>[2x]MSALVLKPCAAVSIRGSSCRARQVAPRAPLAASTVRVALATLEAPARRLGNVACAAAAPAAEAPLSHVQQALAELAKPKDDPTRKHVCVQVAPAVRVAIAETLGLAPGATTPKQLAEGLRRLGFDEVFDTLFGADLTIMEEGSELLHRLTEHLEAHPHSDEPLPMFTSCCPGWIAMLEKSYPDLIPYVSSCKSPQMMLAAMVKSYLAEKKGIAPKDMVMVSIMPCTRKQSEADRDWFCVDADPTLRQLDHVITTVELGNIFKERGINLAELPEGEWDNPMGVGSGAGVLFGTTGGVMEAALRTAYELFTGTPLPRLSLSEVRGMDGIKETNITMVPAPGSKFEELLKH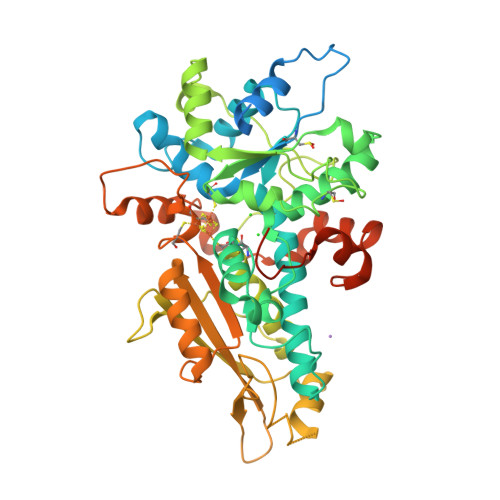RAAARAEAAAHGTPGPLAWDGGAGFTSEDGRGGITLRVAVANGLGNAKKLITKMQAGEAKYDFVEIMACPAGCVGGGGQPRSTDKAITQKRQAALYNLDEKSTLRRSHENPSIRELYDTYLGEPLGHKAHELLHTHYVAGGVEEKDEKKLEIEGRQLGWSHPQFEK>[2x]GHMKLSLSPPPYADAPVVVLISGLGGSGSYWLPQLAVLEQEYQVVCYDQRGTGNNPDTLAEDYSIAQMAAELHQALVAAGIEHYAVVGHALGALVGMQLALDYPASVTVLISVNGWLRINAHTRRCFQVRERLLYSGGAQAWVEAQPLFLYPAD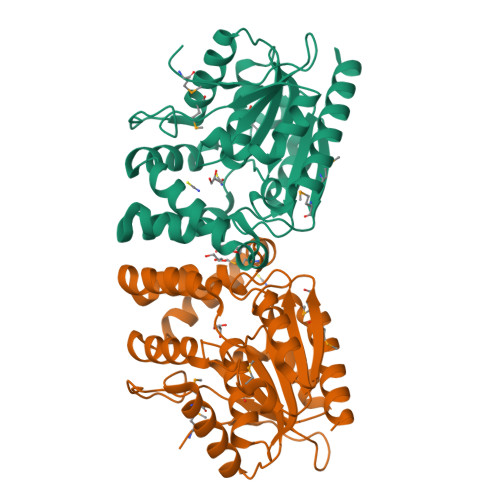WMAARAPRLEAEDALALAHFQGKNNLLRRLNALKRADFSHHADRIRCPVQIICASDDLLVPTACSSELHAALPDSQKMVMPYGGHACNVTDPETFNALLLNGLASLLHHREAAL>[2x]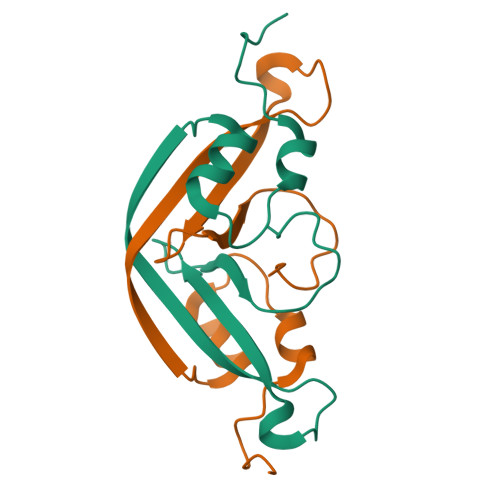SFPGVYKIDIQQGNVVTQDMIDQLRPGMTRRQVRFIMGNPLIVDTFHANRWDYLYSIQPGGGRRQQERVSLFFNDSDQLAGLNGDFMPGVSRDEAILGKEGSTTVTQPADQQKPEAQKEEPPKPGSTLEQLQREVDEAQPVPVPTPEPLDPSPQ>[2x]GPLGSGQYKDNIRHGVCWIYYPDGGSLVGEVNEDGEMTGEKIAYVYPDERTALYGKFIDGEMIEGKLATLMSTEEGRPHFELMPGNSVYHFDKSTSSCISTNALLPDPYESERVYVAESLISSAGEGLFSKVAVGPNTVMSFYNGVRITHQ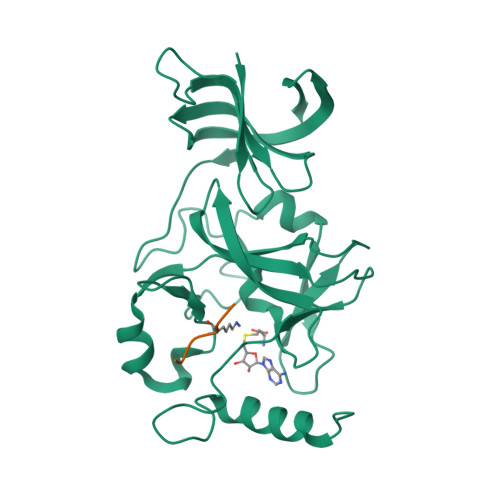EVDSRDWALNGNTLSLDEETVIDVPEPYNHVSKYCASLGHKANHSFTPNCIYDMFVHPRFGPIKCIRTLRAVEADEELTVAYGYDHSPPGKSGPEAPEWYQVELKAFQATQQK;>LKSKKGQSTY[2x]> MSGSMEKLAEIMQEIIEAYQEVKDAFFKFIKAVHEGAPEEELKKYLEKMKEALEKMKELLERLEKEAKKVIEENKDKKLELKVLLMLRLAYLLLKVSIELTKIAAEKLGDKELVEELEKESKEVEKKIKELEE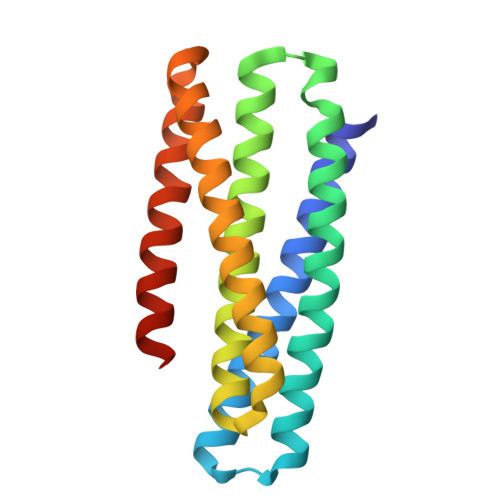RIKKLLEEVDDEELKEAYKEVEEMEKEAEKFLEKMRKVGSG trisulfane | H2 S3 | 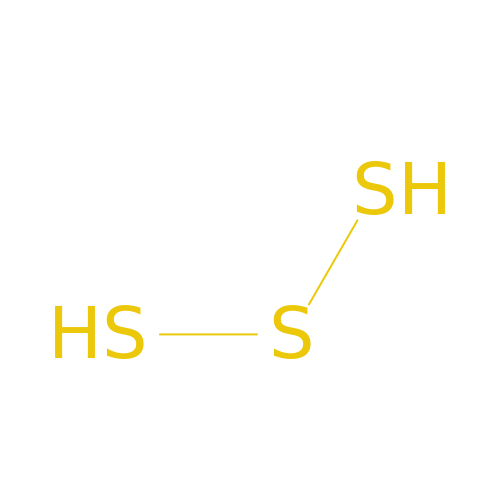KBMBVTRWEAAZEY-UHFFFAOYSA-N> MQVIRKHLAQKGLFNPFLFNRFSTQQDITSVPGDKPPAIEDSIHGKYAGVLFSSASSNKSLNKVAEDMKYFNQLYKESEVFKSFLNNVSLKRNQQRDIISALGKTNFNPATNNLLETLIENKRLDSLPKIAEKYMDYYRILNKQESITIISAQELTAAEKQKVEQGLKKGNANVQFTVVYQVDPAILGGLQMYSGNNFLDCSLLSRVNKLKTEIAKIS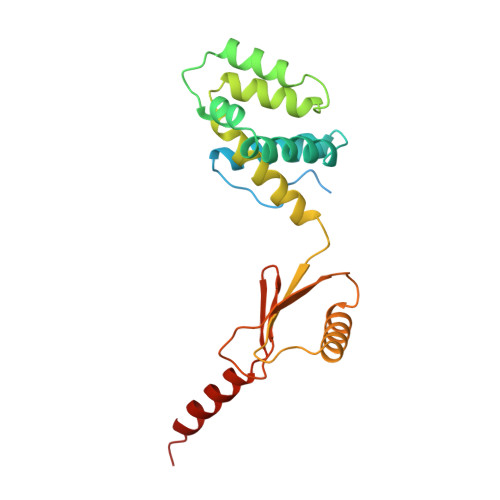F>SIWSRVVQFGTGWGFWVSGHVFITAKHVAPPKGTEIFGRKPGDFTVTSSGDF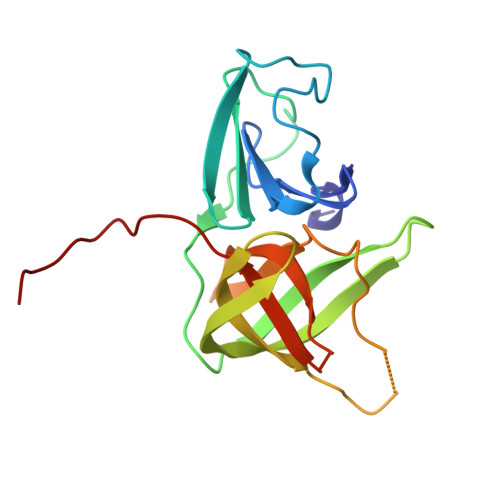LKYYFTSAVRPDIPAMVLENGCQEGVVASVLVKRASGEMLALAVRMGSQAAIKIGSAVVHGQTGMLLTGSNAKAQDLGTIPGDAGCPYVYKKGNTWVVIGVHVAATRSGNTVIAATHGEPTLEAWQA[2x]> SIQGTSLLTQSPASLSTYNDQSVSFVLENGCYVINVDDSGKDQEQDQVLLRYYESPCPASQSGDGVDGKKVMVNMSPIKDTDIWLHANDKDYSVELQRGDVSPPEQAFFVLHKKSSDFVSFECKNLPGTYIGVKDNQLALVEEKDESCNNIMFKLSKI;> AGQRCRFTDVERDKGYTGMLLKGRLRKTAGNGRTVELICGRGNHQYTCESGVLKESSPRQARCGCKGILEMLFDMPKEERPSPMYDSVTYDPTPNTPTTVGKDGIWNGVDYRQGSTVKPYCDTGPVIQGSSKAVCVSGKWVPTLGVCPKMCSIGSLKENGKFVDVTATTKGDELNPPPREQTLIPIVRKVDKDKVQHGVKVVALCKAEDSTTAAEGVQEFECDNGKWKPEPVPCPEP

Interleukin-33 (IL-33) belongs to the IL-1 cytokine family and is an inducer of host allergic and inflammatory responses. The model gastrointestinal nematode Heligmosomoides polygyrus bakeri secretes the Alarmin Release Inhibitor HpARI2, an effector protein that suppresses protective immune responses and asthma in its host by inhibiting IL-33 signalling. HpARI2 is composed of three CCP domains, with CCP1 implicated in DNA binding, while CCP2 and CCP3 are implicated in IL-33 binding. A large loop which emerges from CCP3 directly contacts IL-33 and structural comparison shows that this overlaps with the binding site on IL-33 for its receptor, ST2, preventing formation of a signalling complex.

While crystals containing full-length HpARI2 did not form, crystals were obtained containing the HpARI2_CCP2/3:IL-33 complex and we determined the structure to 2.1 Å. The asymmetric unit of the crystal contained one copy of each of HpARI2_CCP2/3 and mIL-33. The structure of HpARI2_CCP2/3 revealed that the two CCP domains, which are joined by a 3 residue-long linker, are not flexibly associated but instead interact with a buried surface area of 522 Å2. In particular, the 28 residue-long loop which connects strands β5-β6 of CCP3 extends ~28 Å away from CCP3 towards the base of CCP2. IL-33 interacts with both CCP domains of HpARI2_CCP2/3 with a total buried surface area of 1548 Å2. Most of the interaction occurs between the CCP2 domain and the rim of the mIL-33 β-barrel, with a total buried surface area of 1040 Å2 and with contacts involving the edges of β-sheets and interacting side chains. The β-sheet contacts are mediated by main chain hydrogen bonds between CCP2-β1 and β1 of IL-33, which extends the CCP2 domain β-sheet. Residue R159 of IL-33 lies at the centre of this interface and the R159A mutation causes a ~ 1000-fold reduction in binding affinity for HpARI2_CCP2/3. All contacts between IL-33 and HpARI CCP3 are mediated by the long CCP3 loop. Interactions with IL-33 are mostly formed by non-polar residues from, and C-terminal to, a small helix which docks into a small concave, hydrophobic pocket on the top of the mIL-33 β-barrel.> XTDAVLELPAATFDLP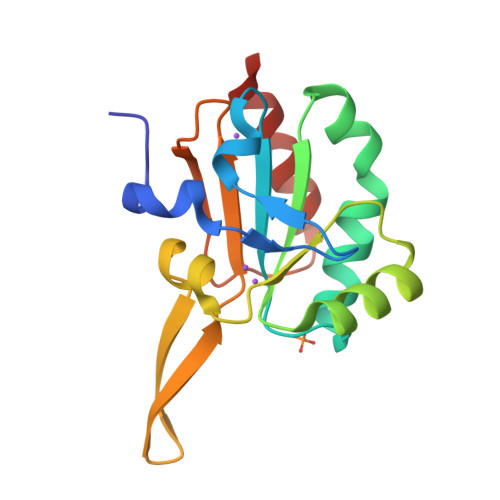LSLSGGTQTTLRAHAGHWLVIYFYPKDSTPGSTTEGLDFNALLPEFDKAGAKILGVSRDSVKSHDNFCAKQGFAFPLVSDGDEALCRAFDVIKEKNMYGKQVLGIERSTFLLSPEGQVVQAWRKVKVAGHADAVLAALKAHAKQ>MNSKCHCVILNDGNFIPVLGFGTALPLECPKSKAKELTKIAIDAGFHHFDSASVYNTEDHVGEAIRSKIADGTVRREDIFYTSKVWCTSLHPELVRASLERSLQKLQFDYVDLYLIHYPMALKPGEENFPVDEHGKLIFDRVDLCATWEAMEKCKDAGLTKSIGVSNFNYRQLEMILNKPGLKYKPVCNQVECHPYLNQMKLLDFCKSKDIVLVAYGVLGTQRDGGWVDQNSPVLLDEPVLGSMAKKYNRTPALIALRYQLQRGIVVLNTSLKEERIKENMQVFEFQLSSEDMKVLDGLNRNM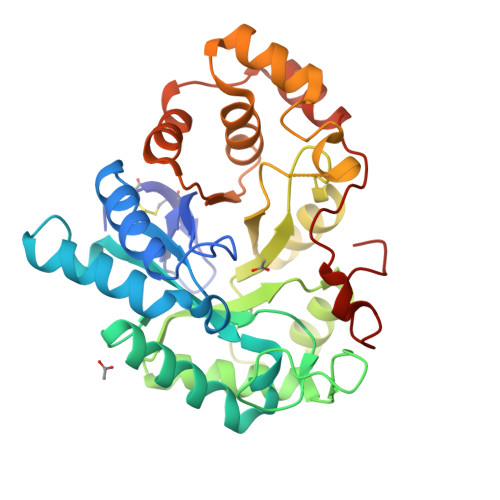RYIPAAIFKGHPNWPFLDEY[2x]>[2x]MAPSQASHTPSLATWTKSLRDQSLEASIESLIFLLKRRQVTGDECAGAIAQLLRQVVAKSKWHDVDQLLYRVQTAGARLARAAPHEPVIGNIVRRVLGLIRDEASENRNADDIASDAASDIQSKSMFNLLSVADPSESPVTGASTPISQAQQPFSVHALRSEVMDGIEEILDEINQADDQIASFAEIQIHPGDYVLAYQPSKTVERFLVKAASKRRFTVILASLNPPAPGEEEQPYAALRK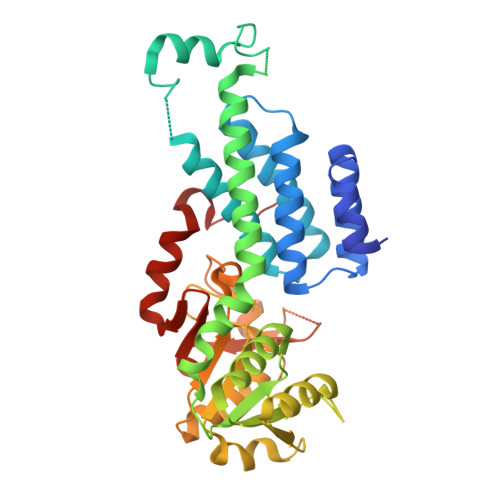KLNAAGVSTINLASNGLMAYIPRVNKVIFGAKAVYQNGGLLVDSGACIAAQAAHEYLKPVIALCGVYKFCPEDPSDEVSRGELGNPSSYVSYADGPELDSFEVENTTTDYIPPDLVDVYLTNLGPQTRHHLGGIYADHYKIEDIGFSLQVGE>MVSKGEEDNMASLPATHELHIFGSINGVDFDMVGQGTGNPNEGYEELNLKSTKGDLQFSPWILVPHVGWGFHQYLPYPDGMSPFQAAMVDGSGYQVHRTMQFEDGASLTVNYRYTYEGSHIKGEAQVKGTGFPADGPVMTNSLTAVDSCWSKKTYPNDKTIISTFKWSYTTGNGERYRSTARTTYTFAKPMAANYLKNQPVYVFRKTELKHSETELNFKEWQKAFTDVMGMDELYK[4x]

mNeonGreen, an engineered green fluorescent protein (GFP) derived from lancelet, is one of the most brightly fluorescent homologs of Aequorea victoria jellyfish GFP (avGFP) yet reported. However, we were ultimately successful in creating a variant, designated as NeonCyan1, with a tryptophan-derived cyan fluorescent protein (CFP)-type chromophore, and two additional mutants with distinct spectral hues. NeonCyan1 has the ‘double humped’ excitation and emission spectra that are characteristic of FPs with Trp-derived chromophores in the neutral state, such as mTurquoise2 and mCerulean3. To obtain insight into the molecular basis of the empirically determined biophysical and photophysical properties of NeonCyan1 and its variants, we determined the crystal structure of NeonCyan0.95 at close to physiological pH (pH 7.5), NeonCyan0.95 at acidic pH (pH 5.6), and NeonCyan1-T207D at close to physiological pH (pH 6.5).

A late-stage variant, designated as NeonCyan0.95 (with Val67Ile rather than Val67Met), was used for structure determination by X-ray crystallography. Inspection of the NeonCyan0.95 crystal structure reveals the locations and interactions of all mutations introduced during directed evolution. Notably, six of the nine mutations appear to be localized in a new dimer interface between monomers A and C of the asymmetric unit. The asymmetric unit contains four molecules of NeonCyan0.95. Calculation of the interaction surfaces between the various monomers (779 Å2 between monomers A and C, 439 Å2 between A and B, 312 Å2 between A and D, 272 Å2 between B and D, 272 Å2 between B and D, and 0 Å2 between B and C) strongly suggests that the symmetrical dimer formed by monomers A and C is physiologically relevant, while other contacts are likely due to crystal packing. The C-terminal MDELYK sequence folds into a helical conformation and contributes to the interaction interface. In the case of NeonCyan0.95 (pH 7.5), the structure revealed the dimer–interface interactions of the protein (discussed next) as well as a water-bridged hydrogen bond network that extended from the indole nitrogen of the chromophore to the hydroxyl group of Thr207. For example, there are two well-defined hydrogen bonds between nitrogen atoms in the chromophore and amino acid side chains. One of these is between a nitrogen atom of the 4-imidazolone ring and the side chain of Glu220, and the other is between the nitrogen atom of the indole ring and a water molecule that is part of a hydrogen bond network that also contains the side chain hydroxyl of Thr207. In addition, one face of the chromophore is closely packed with ionizable residues with side chains potentially bearing positive charges (His72, Lys153, Arg205) and negative charges (Glu45 and Glu220).> GPHMLEQCINPFTNLPHTPRYYDILKKRLQLPVWEYKDRFTDILVRHQSFVLVGETGSGKTTQIPQWCVEYMRSLPGPKRGVACTQPRRVAAMSVAQRVADEMDVMLGQEVGYSIRFEDCSSAKTILKYMTDGMLLREAMNDPLLERYGVIILDEAHERTLATDILMGVLKEVVRQRSDLKVIVMSATLDAGKFQIYFDNCPLLTIPGRTHPVEI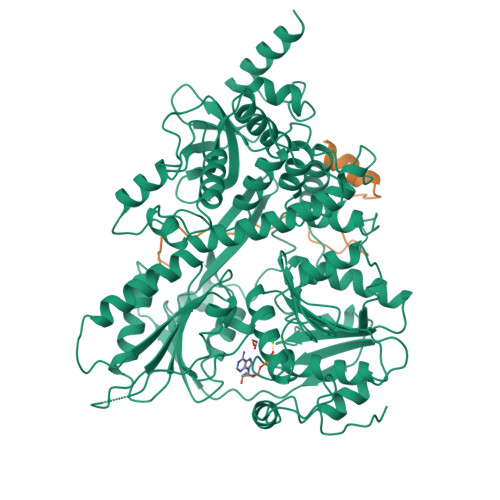FYTPEPERDYLEAAIRTVIQIHMCEEEEGDLLLFLTGQEEIDEACKRIKREVDDLGPEVGDIKIIPLYSTLPPQQQQRIFEPPPPKKQNGAIGRKVVVSTNIAETSLTIDGVVFVIDPGFAKQKVYNPRIRVESLLVTAISKASAQQRAGRAGRTRPGKCFRLYTEKAYKTEMQDNTYPEILRSNLGSVVLQLKKLGIDDLVHFDFMDPPAPETLMRALELLNYLAALNDDGDLTELGSMMAEFPLDPQLAKMVIASCDYNCSNEVLSITAMLSVPQCFVRPTEAKKAADEAKMRFAHIDGDHLTLLNVYHAFKQNHESVQWCYDNFINYRSLMSADNVRQQLSRIMDRFNLPRRSTDFTSRDYYINIRKALVTGYFMQVAHLERTGHYLTVKDNQVVQLHPSTVLDHKPEWVLYNEFVLTTKNYIRTCTDIKPEWLVKIAPQYYDMSNFPQCEAKRQLDRIIAKLQSKEYSQY;> GPHMAEEAYKQQIKEDNIGNQLLRKMGWTGGGLGKSGEGIREPISVKEQHKREGLGLDVERVNKIAK>[2x]LEVQNSCDNCQPGTFCRKYNPVCKSCPPSTFSSIGGQPNCNICRVCAGYFRFKKFCSSTHNAECECIEGFHCLGPQCTRCEKDCRPGQELTKQGCKTCSLGTFNDQAGTGVCRPWTN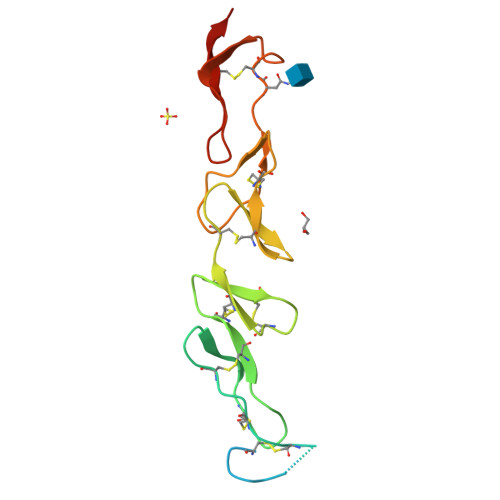CSLDGRSVLKTGTTEKDVVCGPLVPR A single ER‐localised Fic protein, FICD (HYPE), catalyses both AMPylation and deAMPylation of BiP. FICD is a class II Fic protein (with its αinh N‐terminal to its Fic domain) and an ER‐localised type II, single‐pass transmembrane protein, with a short cytoplasmic portion and a large luminal‐facing catalytic domain (Worby et al, 2009; Bunney et al, 2014). We report on the transition of FICD from a dimeric enzyme, that deAMPylates BiP, to a monomer with potent AMPylation activity. Mechanistically, monomerisation relieves a repressive effect allosterically propagated from the dimer interface to the inhibitory Glu234, thereby permitting AMPylation‐competent binding of MgATP.

Co‐expression of reciprocally tagged FICDs confirmed that the wild‐type protein forms homomeric complexes in cells that are disrupted by a previously characterised Leu258Asp mutation within the major dimerisation surface (Bunney et al, 2014). Size‐exclusion chromatography (SEC) and analytical ultracentrifugation (AUC), with purified proteins, confirmed the stability of the FICD dimer (and EV1D–G). These techniques also reaffirmed the strong disrupting effect of the Leu258Asp mutation (in the principal dimer surface) and revealed a weaker disrupting effect of a Gly299Ser mutation (in the secondary dimer surface; Fig EV1D–G). We therefore conclude that between 0.2 and 5 μM (concentrations at which the experiments that follow were performed), the wild‐type protein is dimeric, FICDL258D is monomeric, and FICDG299S is partially monomeric. Complete monomerisation resulted in a 19‐fold increase in AMPylation activity and a 2‐fold decrease in deAMPylation activity. Monomerisation does not result in large conformational changes in FICD. Accordingly, the greatest root‐mean‐squared deviation (RMSD) between the Fic domain of the FICD:ATP structure and any other monomeric or dimer relay FICD structure is 0.53 Å (observed between FICD:ATP and FICDL258D:Apo; residues 213–407). Notably, in all FICD structures the αinh remains firmly juxtaposed to the core Fic domain. In all ATP‐bound structures, the inhibitory glutamate is displaced from the respective apo ground‐state position, in which it forms an inhibitory salt‐bridge with Arg374 (R2 of the Fic motif).

> SLEARAALNQALEMKRQGKREKAQKLFMHALKMDPDFVDALTEFGIFSEEDKDIIQADYLYTRALTISPYHEKALVNRDRTLPLVEEIDQRYFSIIDSKVKKVMSIPKGNSALRRVMEETYYHHIYHTVAIEGNTLTLSEIRHILETRYAVPGKSDEEQNEVIGMHAAMKYINTTLVSRIGSVTISDVLEIHRRVLGYVDPVEAGRFRTTQVLVGHHIPPHPQDVEKQMQEFVQWLNSEEAMNLHPVEFAALAHYKLVYIHPFIDGNGRTSRLLMNLILMQAGYPPITIRKEQRSDYYHVLEAANEGDVRPFIRFIAKCTETTLDTLLFATTEYSVALPEAQP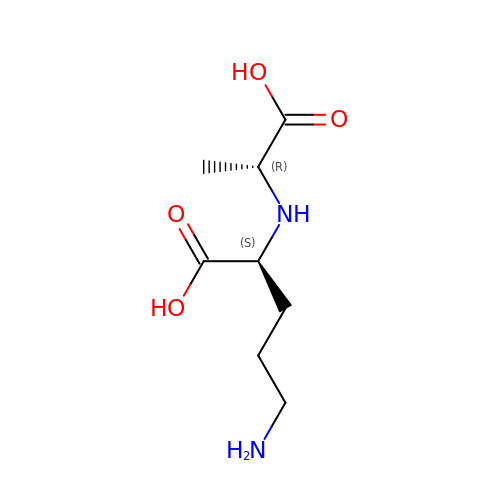(2~{S})-5-azanyl-2-[[(2~{R})-1-oxidanyl-1-oxidanylidene-propan-2-yl]amino]pentanoic acid | C8 H16 N2 O4 | ZQKXJZFWRBQTIO-RITPCOANSA-N>[2x]MQRIIVNPNEPYLSVIKKVVKLSIPIIVVNLLYTVENMISMILVSSISPSAVAATGFSLSLLWFIYSL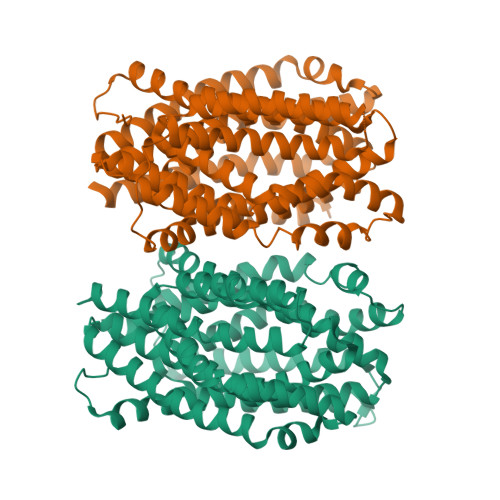MALSYSGTNILIAQFVGAKKDPSPILINGLFLSFLISLPLFFYGKDFVLFLMKVLGASETVRSLAKEYLTPIFWFIPIGFLTNTFYGAYNGAGDTKTPMKVAIIMNLTHIGTAYTLINGKFGLPKLGVEGAGWGIAISEILAFFIYTFLLIFFKKPFPLHLRLEPKLLFKMVRLGTPTALERAITTLSFNVFVGFLAKFGDKVLAAHQIGLRIESISFMIGFGVMIASTTLAGQNYGARNYRGMVHAVNTSAHFTALVMSLTGLILILFPHYLVYPFSRDPEVIEWASYYLQIVGISQPAMAYASIYSGALKGMGKTHIPLFVNISSFWLFRIIPSYFLLKVIHSPLVPWGFMTFETAVRALFYYTVFKKVVGKLLQTFQKEEEPEGEDAEGDKPLDEVRSKVT>VEDATRSDSTTQMSSTPEVVYSSAVDSKQNRTSDFDANWKFMLSDSVQAQDPAFDDSAWQQVDLPHDYSITQKYSQSNEAESAYLPGGTGWYRKSFTIDRDLAGKRIAINFDGVYMNATVWFNGVKLGTHPYGYSPFSFDLTGNAKFGGENTIVVKVENRLPSSRWYSGSGIYRDVTLTVTDGVHVGNNGVAIKTPSLATQNGGNVTMNLTTKVANDTKAAANITLKQTVFPKGGKTDAAIGTVTTASKSIAAGASADVTSTITAASPKLWSIKNPNLYTVRTEVLNGGKVLDTYDTEYGFRWTGFDATSGFSLNGEKVKLKGVSMHHDQGSLGAVANRRAIERQVEILQKMGVNSIRTTHNPAAKALIDVCNEKGVLVVEEVFDMWNRSKNGNTEDYGKWFGQAIAGDNAVLGGDKDETWAKFDLTSTINRDRNAPSVIMWSLGNEMMEGISGSVSGFPATSAKLVAWTKAADSTRPMTYGDNKIKANWNESNTMGDNLTANGGVVGTNYSDGANYDKIRTTHPSWAIYGSETASAINSRGIYNRTTGGAQSSDKQLTSYDNSAVGWGAVASSAWYDVVQRDFVAGTYVWTGFDYLGEPTPWNGTGSGAVGSWPSPKNSYFGIVDTAGFPKDTYYFYQSQWNDDVHTLHILPAWNENVVAKGSGNNVPVVVYTDAAKVKLYFTPKGSTEKRLIGEKSFTKKTTAAGYTYQVYEGADKDSTAHKNMYLTWNVPWAEGTISAEAYDENNRLIPEGSTEGNASVTTTGKAAKLKADADRKTITADGKDLSYIEVDVTDANGHIVPDAANRVTFDVKGAGKLVGVDNGSSPDHDSYQADNRKAFSGKVLAIVQSTKEAGEITVTAKADGLQSSTVKIATTAVPGTSTEKTVRSFYYSRNYYVKTGNKPILPSDVEVRYSDGTSDRQNVTWDAVSDDQIAKAGSFSVAGTVAGQKISVRVTMIDEIGALLNYSASTPVGTPAVLPGSRPAVLPDGTVTSANFAVDWTKPADTVYNTAGTVKVPGTATVFGKEFKV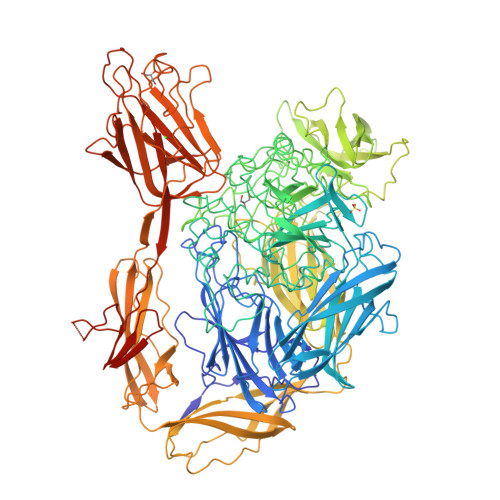TATIRVQRSQVTIGSSVSGNALRLTQNIPADKQSDTLDAIKDGSTTVDANTGGGANPSAWTNWAYSKAGHNTAEITFEYATEQQLGQIVMYFFRDSNAVRFPDAGKTKIQISADGKNWTDLAATETIAAQESSERVKPYTYDFAPVGATFVKVTVTNADTTTPSGVVCAGLTEIELKTATSKFVTNTSAALSSLTVNGTKVSDSVLAAGSYNTPAIIADVKAEGEGNASVTVLPAHDNVIRVITESEDHVTRKTFTINLGTEQEFPADSDERD[6x]>MRSFVLLAFTLSLLAGMSSGPRLNTDYTSANQDSRVQF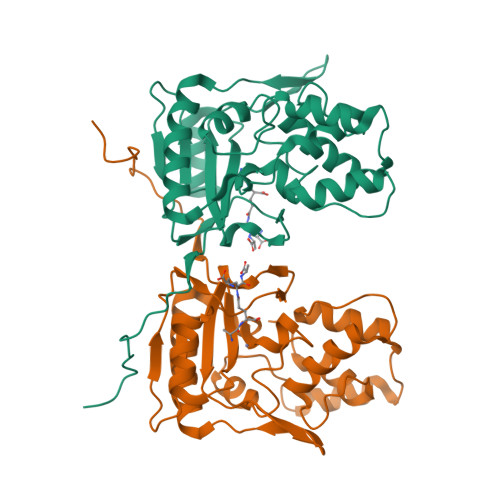IVLHYTSTDLPHSLGILTHGGVSAHYLIGDDEPATVYRLVDENRRAWHAGVSEWQGRTWLNATSIGIEIVNQGYRDTPQGRVWYPFSEAQIQALIPLLKDIAKRHGITPDRIIGHSDIAPGRKVDPGPLFPWKRLADAGLVPWPKPGELARRLAELNGQLPDVRWFQQQLARHGYLVPQTGELEKDTRDVIGAFQMKYRPARFDGEPDLETAALLLAVPTS[2x]> MHHHHHHSSGRENLYFQGNTKNEHHKTNKKSLKGGNERHEMKESSVGISKKIVENSFNNSKLRPGMFIQNSNVVFNEQYKGIKILGKGSFGEVILSRDKHTGHEYAIKVISKKHVKRKTDKESLLREVELLKMLDHINIMKLYEFFEDNNYYYLVSDVYTGGELFDEIISRKRFYEIDAARIIKQILSGITYMHKNNVVHRDLKPENILLETKNKEDMIIKIIDFGLSTHFEYSKKMKDKIGTAYYIAPDVLHGTYDEKCDIWSCGVILYILLSGCPPFNGSNEYDILKKVEAGKYTFDLPQFKKISDKAKDLIKKMLMYTSAVRISARDALEHEWIKMMTSKDNLN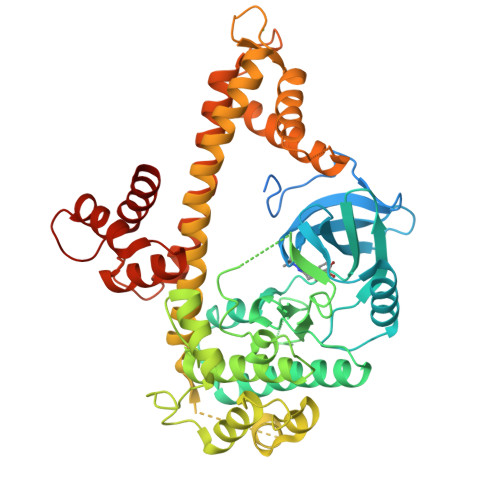IDIPSLELSIANIRQFQSTQKLAQAALLYMGSKLTTIDETKELTKIFKKMDKNGDGQLDRNELIIGYKELLKLKGEDTSDLDNAAIEYEVDQILNSIDLDQNGYIEYSEFLTVSIDRKLLLSTERLEKAFKLFDKDGSGKISANELAQLFGLSDVSSECWKTVLKEVDQNNDGEIDFKEFRDMLVKLCNY>MPGPRIVAFAGSWSRPSKTRSLVEEAARRAVARFGGSAHVFDIADLGPDFGSLRQPQDGPHTRHLDAFLAADALIVASPVYKGSYTGLFKHFIDLIEPVALVGKPVLLAATGGGDRHALVIEHQLRPVFGFFEAHTLATGLYVSASDFGPDGLASEAASTRL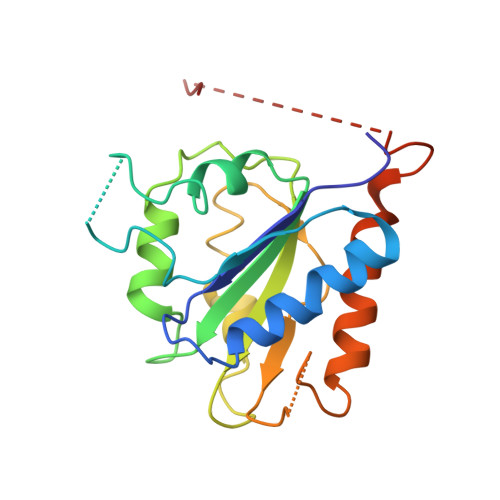DRAVAQFAAHLSRHDAAPLLAVGLEHHHHHH[20x]>MHHHHHHDDDDKTDQEIMDAHKIYFADLNFNPSTGNTYINGMYFAPTQTNKEALDYIQKYRVEATLQYSGFKDIGTKDKEMRNYLGDPNQPKTNYVNLRSYFTGGEN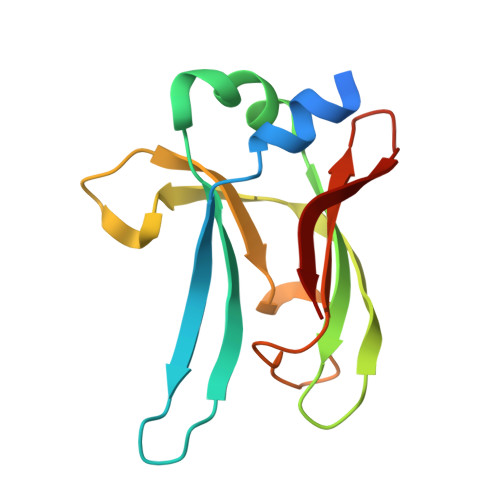IMTYKKLRIYAITPDDRELLVLSVD[2x]>[2x]SMAIRVADLLQHITQMKRGQGYGFKEEYEALPEGQTASWDTAKEDENRNKNRYGNIISYDHSRVRLLVLDGDPHSDYINANYIDGYHRPRHYIATQ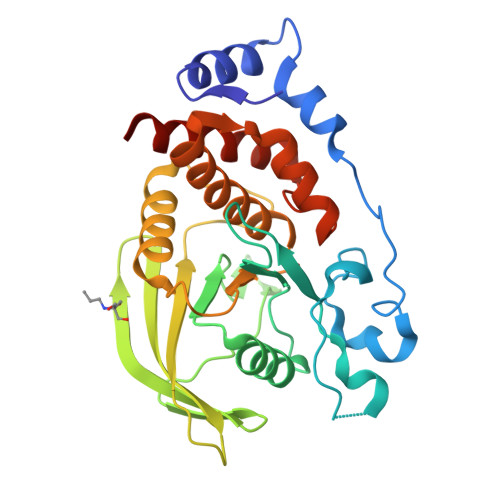GPMQETVKDFWRMIWQENSASIVMVTNLVEVGRVKCVRYWPDDTEVYGDIKVTLIETEPLAEYVIRTFTVQKKGYHEIRELRLFHFTSWPDHGVPCYATGLLGFVRQVKFLNPPEAGPIVVHCSAGAGRTGCFIAIDTMLDMAENEGVVDIFNCVRELRAQRVNLVQTEEQYVFVHDAILEACLCGNTAI4-(4-methyl-1,3-dioxo-1,3-dihydro-2H-isoindol-2-yl)benzonitrile | C16 H10 N2 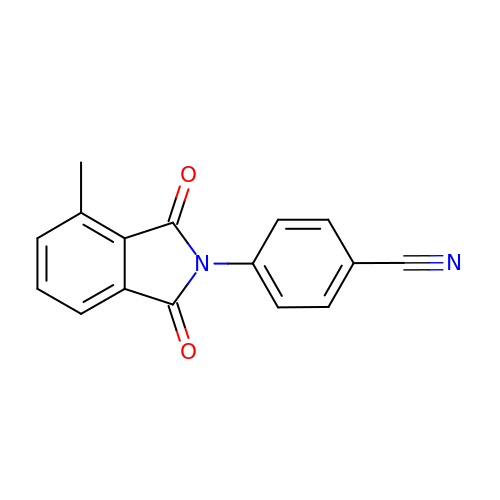O2 | MVYDBJXCIFMINH-UHFFFAOYSA-N>MAHHHHHHVGTFENITAAPADPILGLADLFRADER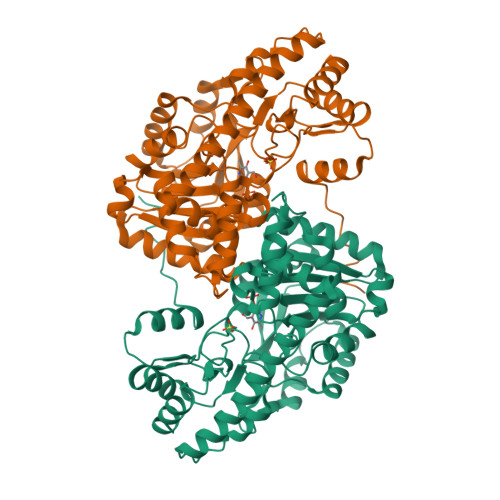PGKINLGIGLYYDETGKIPVLTSVKKAEQYLLENETTKLYLGIDGIPEFGRCTQELLFGKGSALINDKRARTAQTPGGSGALRVAADFLAKNTSVKRVWVSNPSWPNHKSVFNSAGLEVREYAYYDAENHTLDFDALINSLNEAQAGDVVLFHGCCHNPTGIDPTLEQWQTLAQLSVEKGWLPLFDFAYQGFARGLEEDAEGLRAFAAMHKELIVASSYSKNFGLYNERVGACTLVAADSETVDRAFSQMKAAIRANYSSPPAHGASVVATILSNDALRAIWEQELTDMRQRIQRMRQLFVNTLQEKGANRDFSFIIKQNGMFSFSGLTKEQVLRLREEFGVYAVASGRVNVAGMTPDNMAPLCEAIVAVL[2x]>[2x]MGHHHHHHGSMSQNVYIVSTARTPIGSFQGSLS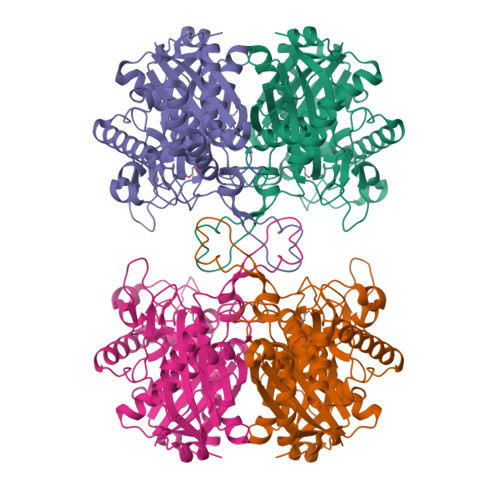SKTAVELGAVALKGALAKVPELDASKDFDEIIFGNVLSANLGQAPARQVALAAGLSNHIVASTVNKVAASAMKAIILGAQSIKCGNADVVVAGGCESMTNAPYYMPAARAGAKFGQTVLVDGVERDGLNDAYDGLAMGVHAEKCARDWDITREQQDNFAIESYQKSQKSQKEGKFDNEIVPVTIKGFRGKPDTQVTKDEEPARLHVEKLRSARTVFQKENGTVTAANASPINDGAAAVILVSEKVLKEKNLKPLAIIKGWGEAAHQPADFTWAPSLAVPKALKHAGIEDINSVDYFEFNEAFSVVGLVNTKILKLDPSKVNVYGGAVALGHPLGCSGARVVVTLLSILQQEGGKIGVAAICNGGGGASSIVIEKI>[6x]LREQPQQNECQLERLDALEPDNRIESEGGLIETWNPNNKQFRCAGVALSRATLQRNALRRPYYSNAPQEIFIQQGNGYFGMVFPGCPETFEEPQESEQGEGRRYRDRHQKVNRFREGDIIAVPTGIVFWMYNDQDTPVIAVSLTDIRSSNNQLDQMPRRFYLAGNHEQEFLQYQHQQGGKQEQENEGNNIFSGFKRDFLEDAFNVNRHIVDRLQGRNEDEEKGAIVKV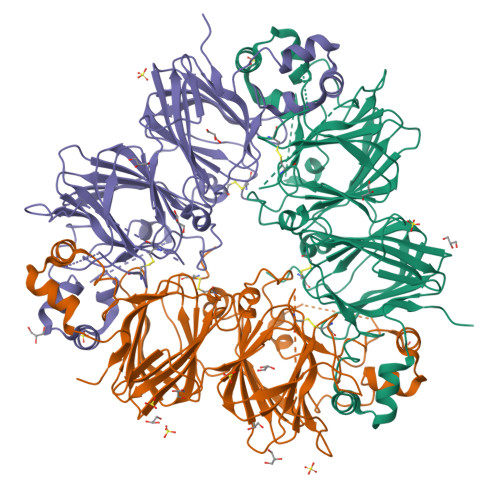KGGLSIISPPEKQARHQRGSRQEEDEDEEKQPRHQRGSRQEEEEDEDEERQPRHQRRRGEEEEEDKKERGGSQKGKSRRQGDNGLEETVCTAKLRLNIGPSSSPDIYNPEAGRIKTVTSLDLPVLRWLKLSAEHGSLHKNAMFVPHYNLNANSIIYALKGRARLQVVNCNGNTVFDGELEAGRALTVPQNYAVAAKSLSDRFSYVAFKTNDRAGIARLAGTSSVINNLPLDVVAATFNLQRNEARQLKSNNPFKFLVPARESENRASA> GAMGKVTHSIHIEKSDTAADTYGFSLSSVEEDGIRRLYVNSVKETGLASKKGLKAGDEILEINNRAADALNSSMLKDFL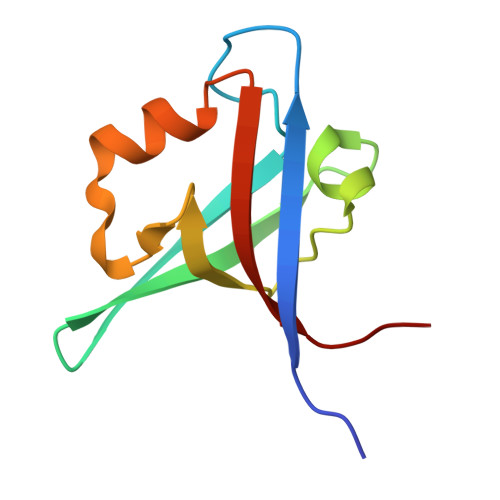SQPSLGLLVRTYPEL> GSKTISESELSASATELLQDYMLTLRTKLSSQEIQQFAALLHEYRNGASIHEFCINLRQLYGDSRKFLL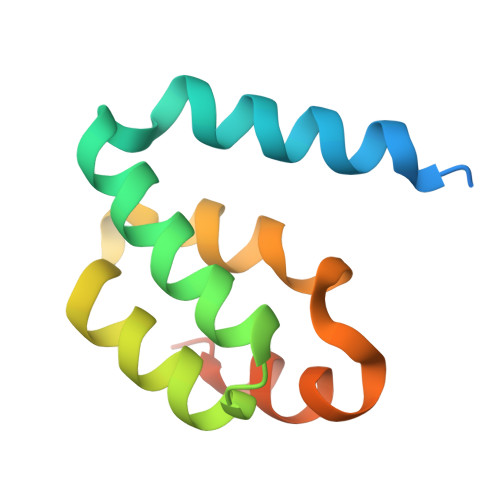LGLRPFIPEKDSQHFENFLETIGVKDGRG> MPKPINVRVTTM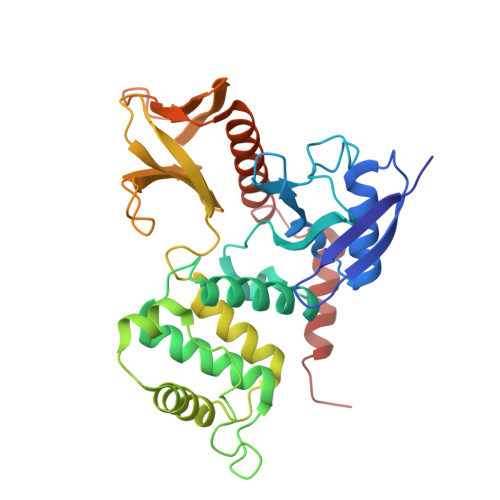DAELEFAIQPNTTGKQLFDQVVKTVGLREVWFFGLQYVDSKGYSTWLKLNKKVTQQDVKKENPLQFKFRAKFFPEDVSEELIQEITQRLFFLQVKEAILNDEIYCPPETAVLLASYAVQAKYGDYNKEIHKPGYLANDRLLPQRVLEQHKLTKEQWEERIQNWHEEHRGMLREDSMMEYLKIAQDLEMYGVNYFEIKNKKGTELWLGVDALGLNIYEHDDKLTPKIGFPWSEIRNISFNDKKFVIKPIDKKAPDFVFYAPRLRINKRILALCMGNHELYMRRRKPDTIEVQQMKAQARVDSSGAA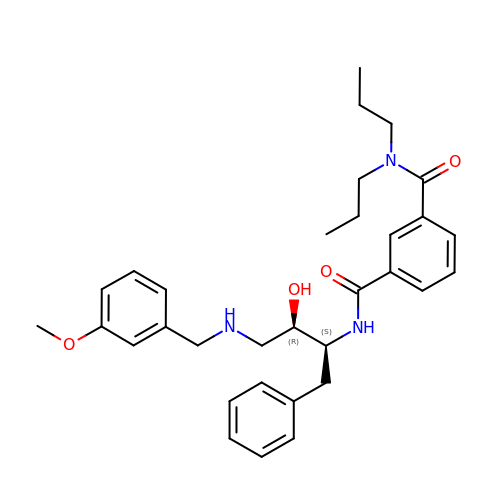3-[({(1S,2R)-1-BENZYL-2-HYDROXY-3-[(3-METHOXYBENZYL)AMINO]PROPYL}AMINO)(HYDROXY)METHYL]-N,N-DIPROPYLBENZAMIDE | C32 H41 N3 O4 | WPRACYICKOKGTO-XZWHSSHBSA-N> PALTKSQTDRLEVLLNPKDEISLNSGKPFRELESELLSRRKKDLQQIYAEERENYLGKLEREITRFFVDRGFLEIKSPILIPLEYIERMGIDNDTELSKQIFRVDKNFCLRPMVAPNIFNYARKLDRALPDPIKIFEIGPCYRKESDGKEHLEEFTMLNFFQMGSGCTRENLESIITDFLNHLGIDFKIVGDSCSVYGDTLDVMHGDLEL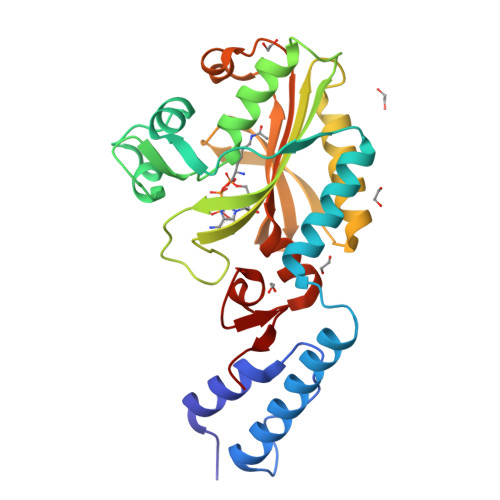SSAVVGPIPLDREWGIDKPWIGAGFGLERLLKVKHDFKNIKRAARSESYYNGISTNL PHTHALIC ACID | C8 H6 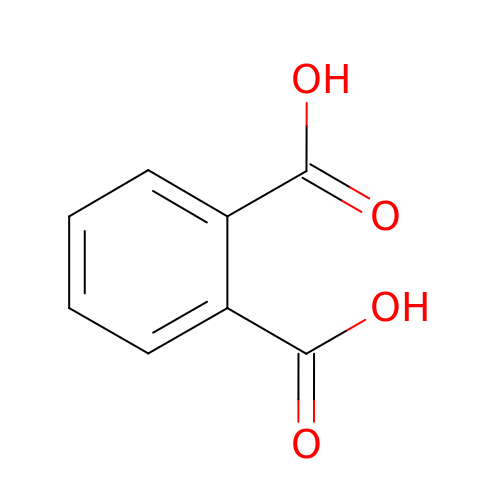O4 | XNGIFLGASWRNHJ-UHFFFAOYSA-N>GMSTFRQEDVEDHYEMGEELGSGQFAIVRKCRQKGTGKEYAAKFIKKRRLSSSRRGVSREEIEREVNILREIRHPNIITLHDIFENKTDVVLILELVSGGELFDFLAEKESLTEDEATQFLKQILDGVHYLHSKRIAHFDLKPENIMLLDKNVPNPRIKLIDFGIAHKIEAGNEFKNIFGTPEFVAPEIVNYEPLGLEADMWSIGVITYILLSGASPFLGETKQETLTNISAVNYDFDEEYFSNTSELAKDFIRRLLVKDPKRRMTIAQSLEHSWIKA[2x]

Members of the DAPK family are generally involved in both apoptotic and autophagy pathways and share significant overall sequence similarity with myosin light chain-related kinases and triple functional domain protein-related kinases (Temmerman et al., 2013). DAPK1 and DAPK2 bind Ca2+/CaM through a closely related ARD, which is inhibited by phosphorylation of an identical ARD residue Ser308 in both kinases (Shani et al., 2001, Shohat et al., 2001). They also contain a basic loop (BL) in the kinase N lobe next to the kinase active site, which has been identified as a DAPK-family-specific signature motif (Tereshko et al., 2001). We found an identical type of dimer arrangement in all three kinases that involves the BL of the CD. In terms of functional implications, CD dimerization in hDAPK1, hDAPK2, and hDAPK3 is likely to inhibit catalytic activity by directly occluding the kinase active site.

Since hDAPK3 has no ARD, the hDAPK3 construct we used was limited to the CD. All three kinases were crystallized and the resulting structures were refined to a resolution of 2.0 Å (hDAPK1), 1.47 Å (hDAPK2), and 3.1 Å (hDAPK3). The root-mean-square deviation (RMSD) values of superimposed dimers from the different hDAPKs are in the range of 1.2–2.0 Å, demonstrating that the type of dimerization observed in the structures of hDAPK1, hDAPK2, and hDAPK3 is conserved. The second main dimer interface is formed from positively charged residues on the DAPK signature BL segment, which belongs to the most mobile areas in the DAPK structures. In the DAPK3 structure, in which the BL residue 50 is a serine instead of an arginine, the most specific interactions are formed by Arg53 and residues C-terminal to the BL from helix αC: Ser57 and Glu60. In DAPK3 there is an additional specific interaction with Glu182, which is the central residue of the PEF/Y motif and a key contributor to DAPK substrate recognition (Temmerman et al., 2014). For DAPK3, canonical kinase domain-mediated homodimeric assembly via activation loop swapping has been reported (Pike et al., 2008).> MRYEDRVIFQLEQVATYNPKTSKKENTLITYDAIPCNINPISRAR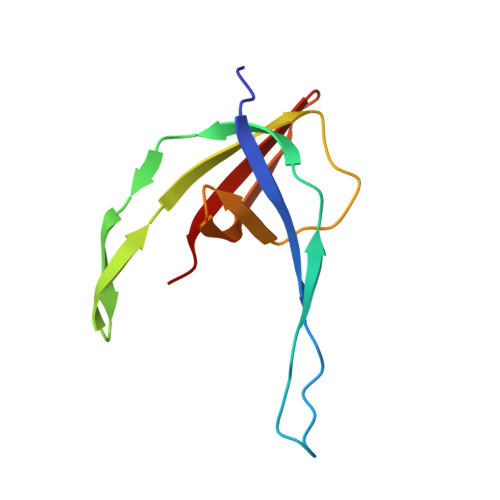KQLEFGDVKNDVSVLRIKESISYPVSHVLVNGIRYKIVDTRIYRHETSYYIEEVN> RSVYELDCIPLWGVVSIQGNRSEMEDAFAVSPHFLKLPIKMLMGDHEGMSPSLTHLTGHFFGVYDGHGGHKVADYCRDRLHFALAEEIERIKDELCKRNTGAGRQVQWDKVFTSCFLTVDGEIEGKIGRAVVGSSDKVL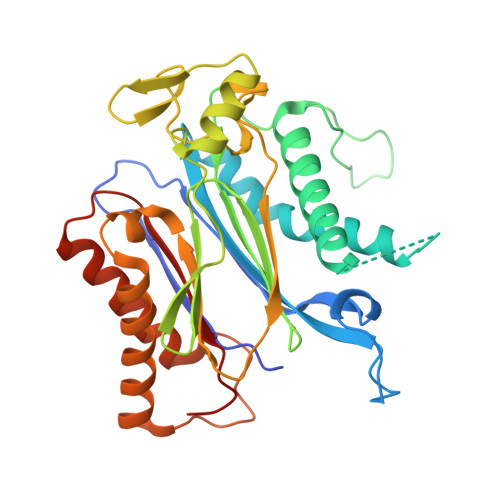EAVASETVGSTAVVALVCSSHIVVSNCGDSRAVLFRGKEAMPLSVDHKPDREDEYARIENAGGKVIQWQGARVFGVLAMSRSIGDRYLKPYVIPEPEVTFMPRSREDECLILASDGLWDVMNNQEVCEIARRRILMWHKKNGAPPLAERGKGIDPACQAAADYLSMLALQKGSKDNISIIVIDLKAQRKFKTRT>[3x]SPKPFTFEAGERAVLLLHGFTGNSSDVRMLGRFLESKGYTCHAPIYKGHGVPPEELVHTGPD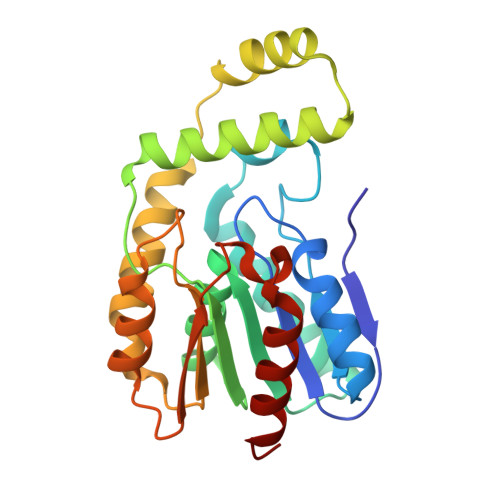DWWQDVMNAYEFLREKGYQKIAVVGLSLGGVFSLKLGYTVPVVGIVPMCAPMYIKSEETMYQGVLDYAREYKKREGKAPEQIEKEMEEFRKTPMKTLKALQALIAEVRNHIDLIYAPTFVVQARHDDMINTDSANIIYNGVESPIKQIKWYEESGHVITLDKEKEQLHEDIYAFLESLDW> MASWSHPQFEKGASTSLYKKAGSAAAVLEENLYFQGSFTAKMAFTLADRVTEEMLADKAALVVEVVEENYHDAPIVGIAVVNEHGRFFLRPETALADPQFVAWLGDETKKKSMFDSKRAAVALKWKGIELCGVSFDLLLAAYLLD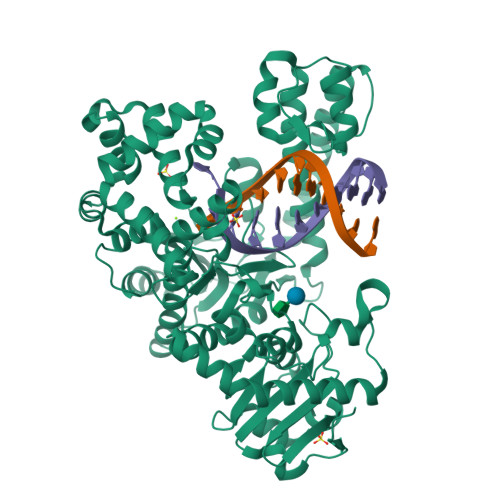PAQGVDDVAAAAKMKQYEAVRPDEAVYGKGAKRAVPDEPVLAEHLVRKAAAIWALERPFLDELRRNEQDRLLVELEQPLSSILAEMEFAGVKVDTKRLEQMGEELAEQLRTVEQRIYELAGQEFNINSPKQLGVILFEKLQLPVLKKSKTGYSTSADVLEKLAPYHEIVENILHYRQLGKLQSTYIEGLLKVVRPDTKKVHTIFNQALTQTGRLSSTEPNLQNIPIRLEEGRKIRQAFVPSESDWLIFAADYSQIELRVLAHIAEDDNLMEAFRRDLDIHTKTAMDIFQVSEDEVTPNMRRQAKAVNFGIVYGISDYGLAQNLNISRKEAAEFIERYFESFPGVKRYMENIVQEAKQKGYVTTLLHRRRYLPDITSRNFNVRSFAERMAMNTPIQGSAADIIKKAMIDLNARLKEERLQARLLLQVHDELILEAPKEEMERLCRLVPEVMEQAVTLRVPLKVDYHYGSTWYDAK> APKAPADGLKMDKTKQPVVFNHSVHKAVKCGDCHHPVNGKEDYQKCATAGCHDNMDKKDKSAKGYYHAMH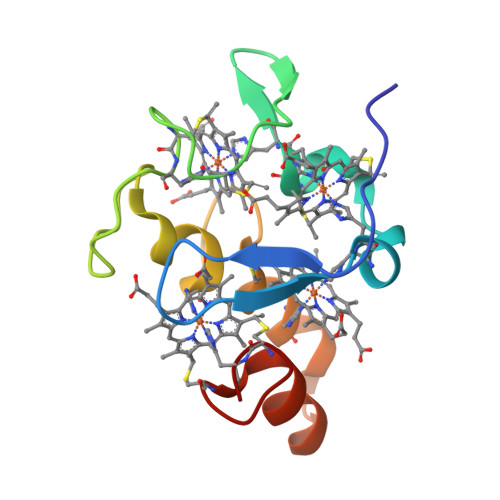DKGTKFKSCVGCHLETAGADAAKKKELTGCKGSKCHS> ENSLEIEELARFAVDEHNKKENALLEFVRVVKAKEQMFSWLDWEETMYYLTLEAKDGGKK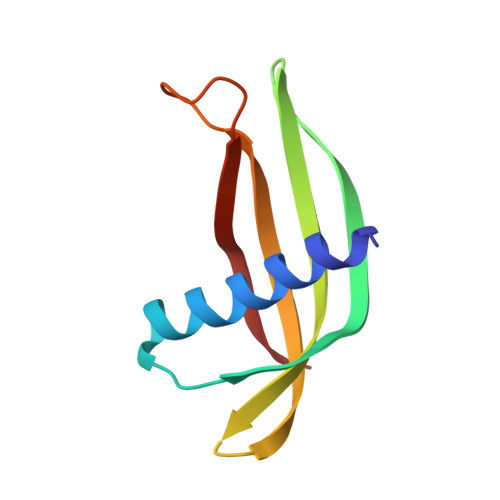KLYEAKVWVKPALLWSPHGNFKELQEFKPV>AVPETRPNHTIYINNLNEKIKKDELKKSLHAIFSRFGQILDILVSRSLKMRGQAFVIFKEVSSATNALRSMQGFPFYDKPMRIQYAKTDSDIIA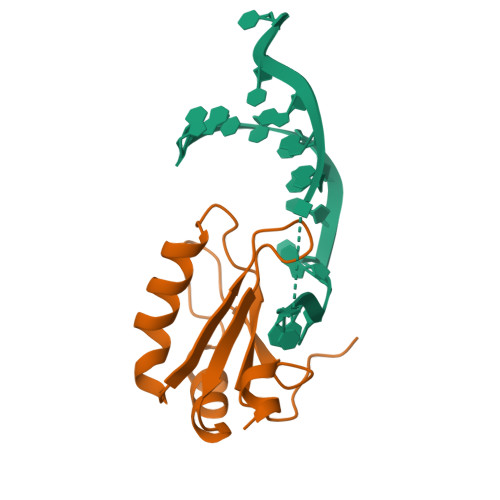KMK[3x]>[2x]HGYVSAVENGVAEGRVTLCKFAANGTGEKNTHCGAIQYEPQSVEGPDGFPVTGPRDGKIASAESALAAALDEQTADRWVKRPIQAGPQTFEWTFTANHVTKDWKYYITKPNWNPNQPLSRDAFDLNPFCVVEGNMVQPPKRVSHECIVPEREGYQVILAVWDVGDTAASFYNVIDVKFDGNGPVLPDWNPAGQIIPSMDLSIGDTVYTRVFDNDGENPAYRTELKIDSET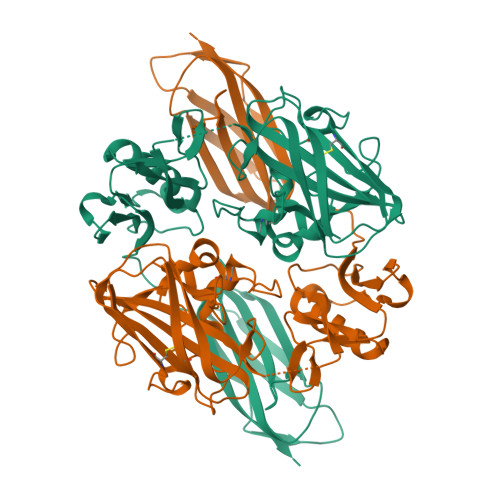LTKANQWSYALATKINQTQKQQRAGQLNGDQFVPVYGTNPIYLKEGSGLKSVEIGYQIEAPQPEYSLTVSGLAKEYEIGEQPIQLDLTLEAQGEMSAELTVYNHHQKPLASWSQAMTDGELKSITLELSEAKAGHHMLVSRIKDRDGNLQDQQTLDFMLVE>MAHHHHHHMSERVILAYSGGLDTSVAISWIGKETGREVVAVAIDLGQGGEDMEVVRQRALDCGAVESIVIDARDEFANDYCVPAIQSNALYMDRYPLVSALSRPLIVKHLVKAAREHGGTIVAHGCTGKGNDQVRFEVGFASLAPDLEVLAPVRDYAWTREKAIAFAEENNIPINVTKRSPFSIDQNVWGRAVETGFLEHLWNAPTKDVYSYTEDPTVNWSTPDEVIVGFEQGVPVSIDGRSVTPLQAIEELNRR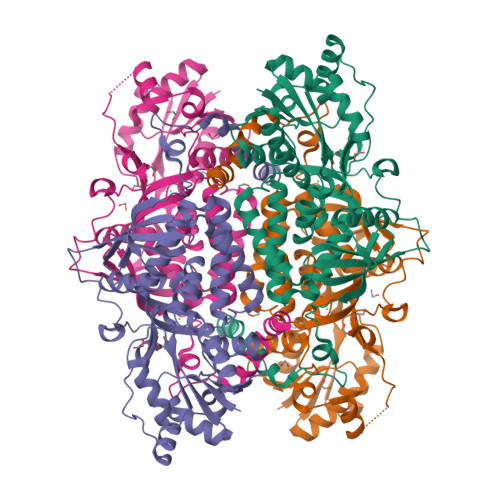GGEQGVGRLDVVEDRLVGIKSREIYEAPGAMVLITAHTELEHVTLERELGRFKRITDQKWGELVYDGLWFSPLKTALESFVAKTQEHVTGEIRMVLHGGHIAVNGRRSPKSLYDFNLATYDEGDTFDQSAAKGFVQIHGLSSSISARRDLQGQ[2x]>MAEDIPSLAEAFRDYFPIGAAIEPGYTTGQIAELYKKHVNMLVAENAMKPASLQPTEGNFQWADADRIVQFAKENGMELRFHTLVWHNQTPDWFFLDKEGKPMVEETDPQKREENRKLLLQRLENYIRAVVLRYKDDIKSWDVVNEVIEPNDPGGMRNSPWYQITGTEYIEVAFRATREAGGSDIKLYINDYNTDDPVKRDILYELVKNLLEKGVPIDGVGHQTHIDIYNPPVERIIESIKKFAGLGLDNIITELDMSIYSWNDRSDYGDSIPDYILTL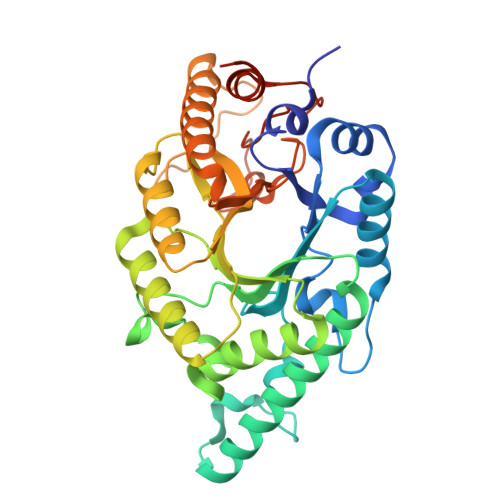QAKRYQELFDALKENKDIVSAVVFWGISDKYSWLNGFPVKRTNAPLLFDRNFMPKPAFWAIVDPSRLRELEHHHHHH[2x]4-amino-1-[(2R,3R,4S,5R)-3,4-dihydroxy-5-(hydroxymethyl)oxolan-2-yl]-5-fluoro-pyrimidin-2-one 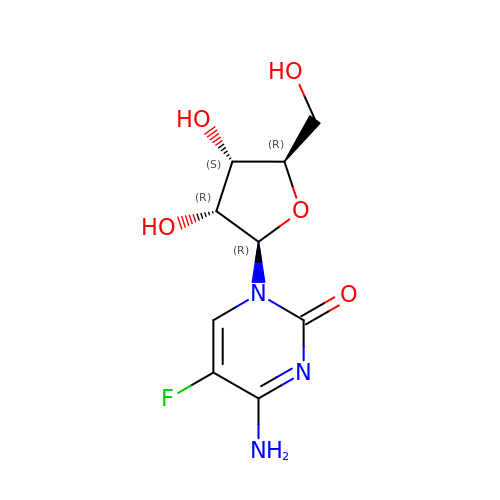| C9 H12 F N3 O5 | STRZQWQNZQMHQR-UAKXSSHOSA-N>[4x]MRIIMPVEFSRIVRDVERLIAVEKYSLQGVVDGDKLLVVGFSEGSVNAYLYDGGETVKLNREPINSVLDPHYGVGRVILVRDVSKGAEQHALFKVNTSRPGEEQRLEAVKPMRILSGVDTGEAVVFTGATEDRVALYALDGGGLRELARLPGFGFVSDIRGDLIAGLGFFGGGRVSLFTSNLSSGGLRVFDSGEGSFSSASISPGMKVTAGLETAREARLVTVDPRDGSVEDLELPSKDFSSYRPTAITWLGYLPDGRLAVVARREGRSAVFIDGERVEAPQGNHGRVVLWRGKLVTSHTSLSTPPRIVSLPSGEPLLEGGLPEDLRRSIAGSRLVWVESFDGSRVPTYVLE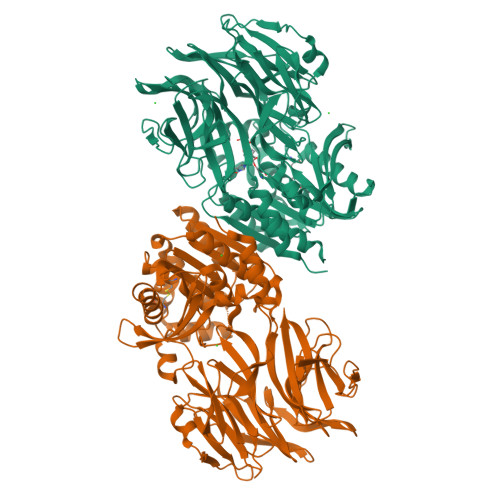SGRAPTPGPTVVLVHGGPFAEDSDSWDTFAASLAAAGFHVVMPNYRGSTGYGEEWRLKIIGDPCGGELEDVSAAARWARESGLASELYIMGYSYGGYMTLCALTMKPGLFKAGVAGASVVDWEEMYELSDAAFRNFIEQLTGGSREIMRSRSPINHVDRIKEPLALIHPQNDSRTPLKPLLRLMGELLARGKTFEAHIIPDAGHAINTMEDAVKILLPAVFFLATQRERR> QGVRTFVDPFTFEDPNQAVREFAKEIDASCIKIEKVIGVGEFGEVCSGRLKVPGKREICVAIKTLKAGYTDKQRRDFLSEASIMGQFDHPNIIHLEGVVTKCKPVMIITEYMENGSLDAFLRKNDGRFTVIQLVGMLRGIGSGMKYLSDMSAVHRDLAARNILVNSNLVCKVSDFGMSRVLED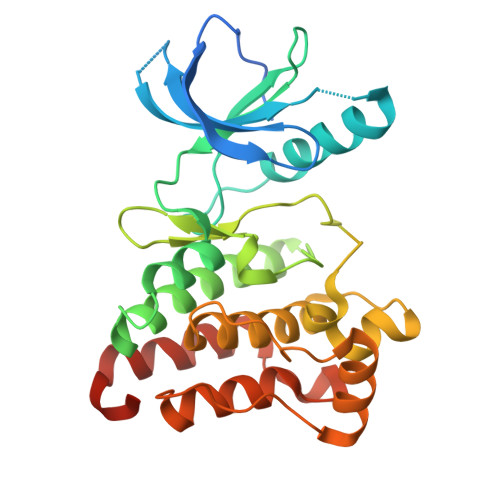DPEAAYTTRGGKIPIRWTAPEAIAYRKFTSASDVWSYGIVMWEVMSYGERPYWDMSNQDVIKAIEEGYRLPPPMDCPIALHQLMLDCWQKERSDRPKFGQIVNMLDKLIRNPNSLKRTGSESS Here, we conduct a comprehensive functional analysis of the Antibiotic_NAT family of aminoglycoside acetyltransferases. AG resistance is primarily conferred by three classes of aminoglycoside-modifying enzymes (AMEs): phosphotransferases (APHs), nucleotidylyltransferases (ANTs), and acetyltransferases (AACs). AMEs permanently alter the AG substrate, preventing them from binding to their target, the A-site of the 16S rRNA in the bacterial ribosome. The fold typical of the Antibiotic_NAT family is evident in all structures, composed of 13 α-helices and 8 β-strands, and determined structures superpose with pairwise RMSD’s 0.8–1.0 Å between 197 to 266 matching Cα atoms.

To increase the chances of capturing substrate-bound enzyme complex we used the catalytically impaired His154Ala mutant of AAC(3)-IVa. Using this strategy, we were able to determine the crystal structures of AAC(3)-IVa enzyme in complex with gentamicin or apramycin to 2.6 and 2.8 Å, respectively. In both complex structures, the electron density corresponding to the AG molecule localized to the cleft between the major and minor subdomains of the enzyme. For the AG substrate in both structures, the 3-N group is positioned close to residue 154 and proximal to the presumed location of the thiol of CoA. In the complex structures, the gentamicin molecule spans across the enzyme’s minor subdomain while the apramycin molecule is twisted nearly 90° relative to gentamicin. This difference is reflected in the rotation of the 2-deoxystreptamine rings of each compound. The 2-deoxystreptamine/II ring of apramycin stacks against the sidechain of Trp63, and its rotation positioned the central and III rings more into the minor subdomain cleft and towards Asp67. Notably, these two residues are contributed from the much shorter hairpin connecting the α4 and α5 helices compared to the equivalent region in the other enzymes we crystallized. Additionally, Glu185 appears to be a critical residue for interactions with gentamicin and apramycin as it positions the 2-deoxystreptamine ring for modification through interactions with the 1-N of gentamicin or the 5-hydroxyl of apramycin. Finally, the C-terminal extension of AAC(3)-IVa corresponding to residues 236-257 contributes to the interactions with both gentamicin and apramycin via Glu249 side chain.

>QGMQYEWRKAELIGQLLNLGVTPGGVLLVHSSFRSVRPLEDGPLGLIEALRAALGPGGTLVMPSWSGLDDEPFDPATSPVTPDLGVVSDTFWRLPNVKRSAHPFAFAAAGPQAEQIISDPLPLPPHSPASPVARVHELDGQVLLLGVGHDANTTLALAELMAKVPYGVPRHCTILQDGKLVRVDYLENDHCCERFALADRWLKEKSLQKEGPVGHAFARLIRSRDIVATALGQLGRDPLIFLHPPEAGCEECDAARQSIG[6x]> MVRRSHVVAYYWSRYRMPTQMPKFDGPAPVAAPQSMNSTKTNEFIDPIDDKFPMSIRGPLVRPDVPEDQYVDSWYICTSMTHHMGDYRPWSASAPPNAFRFRPFNEFDAKGREYVQYMREFARFDPRKSRGNGQKGFPFRDAYLTKMNEANQKTPPPTLETIMDRAVREHHQHARILSPLEVQRDVGRLEPIPSYAGKINADRSVFPFQWKTEDWYEYEVAKVRNRRFVFENTEEDGIRGSEVTYKIVLEGFWDHHVMKLAEDVCMFLKDVGRQIVEEKLVAVRRLLQGGAVDPELLAAFNCARAGP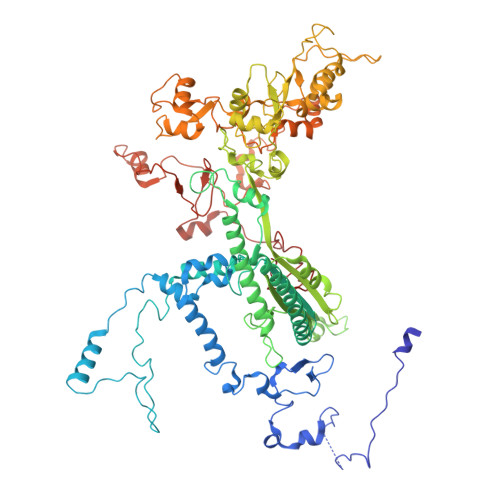FGGLDEYDKEEVANFLRSDLRRLEEQCLSVINRCNVPVPGATNIYDPHTSWPHVEKLEPWVRMAEFWTSSSDTSFTELEMSTAHYEFRKFFRVIICKLPFQSTEFEKRMYDIRHWLHRQTSCEFHTIYRRNVIHDSAVFPTEHDPATPTTHEHHRMFSFALDWQSAPVNRLSTDTVHEGESWDAVAQRLGCSVGELKDANAERETIEAGVVINVPVTATRRLTSFGATPLVLPLKTTSAKDGERIRTWEEAAAILDCTVEELQQCNGHAALTYQKKESEAGEFDSSVTELVAPLSCWTSTSESEFSPVERVHANDTLVAIARRLQCSEEALRAVNDGITDVSGLDFVRVPPEARRPRRLVEPQLRPQAATDALLARTIAEEETFKLKSIPHLPQNAERFPHEYHTPTSRFPPTPSETPATQDWMAYTAKYLDKQFTISAEPAPVYNVNKLWPMQQIPGKVDQTPFEEDQTWLLHSIPVQQLEMHHHEKDLQDLPFINHEQFPRSLEWNAP>[3x]MAHHHHHHSSGLEVLFQGPMTHSVVELIEIESAIIQVKMQDRTHKNAFSQELTDDLIQAFEYIRQNPKYKAVILTGYDNYFASGGTQEGLLRIQQGLTKFTDDNLYSLALDCEIPVIAAMQGHGIGGGFVMGLFADIVILSRESVYTANFMKYGFTPGMGATFIVPKKLGFSLAQEILLNAGSYRGADLEKRGVPFKVLPRAEVLDYAVELAQELAEKPRNSLVTLKDHLVAPLRDQLPRVIEQELMMHEKTFHHEEVKSRIKGLYGN

In this study we present a structural and functional description of the bacillaene synthase β-branching enzymes PksH and PksI. These biocatalysts are responsible for the final two steps in β-methyl branch incorporation in this PKS/NRPS pathway. There is a single active site per PksI monomer, with each active site positioned on the periphery of the trimer, ~ 43 Å from one other. Akin to PksH, PksI adopts a characteristic CS fold, with a ββα core, that comprises two approximately perpendicular -sheets surrounded by -helices.

Two crystal structures of PksI were elucidated; the first to 1.93 Å resolution using a crystal cryoprotected in glycerol (PksI_GOL), and the second to 2.1 Å using a crystal cryoprotected using ethylene glycol (PksI_EG). Both structures describe an asymmetric unit comprised of three protein chains arranged in the form of a trimer. The final model of PksI_EG comprises residues 1–248 of chain A, residues 2–248 of chain B, and residues 4–232 of chain C, 417 water molecules, 4 molecules of ethylene glycol and 2 molecules of glycerol. In the PksI_EG structure all the active sites adopt the “closed” ground state conformation. In the absence of bound ligand, the PksI active site adopts an “closed” conformation, where the side chains of residues Phe81 and Phe136 occupy the central solvent exposed cavity of the enzyme active site. In this state the catalytic residue His230 is found to point away from the centre of the site in an apparent catalytically incompetent conformation.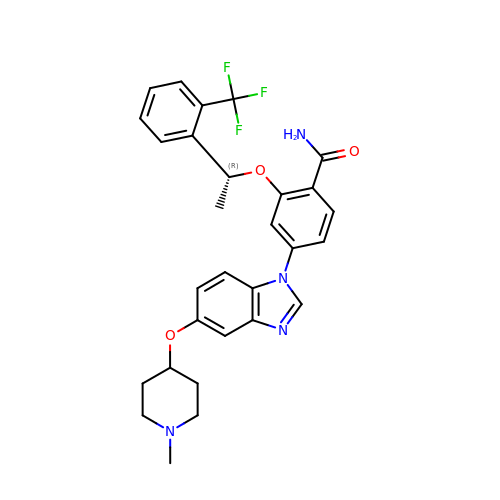4-{5-[(1-METHYLPIPERIDIN-4-YL)OXY]-1H-BENZIMIDAZOL-1-YL}-2-{(1R)-1-[2-(TRIFLUOROMETHYL)PHENYL]ETHOXY}BENZAMIDE | C29 H29 F3 N4 O3 | FASALJZFFLCNKM-GOSISDBHSA-N>SIAGITEPTILQYFATLNAGEFAATAALFAVDGVMYPPFESGIVGPDAIAAYLQQEAQGIKAEPQQ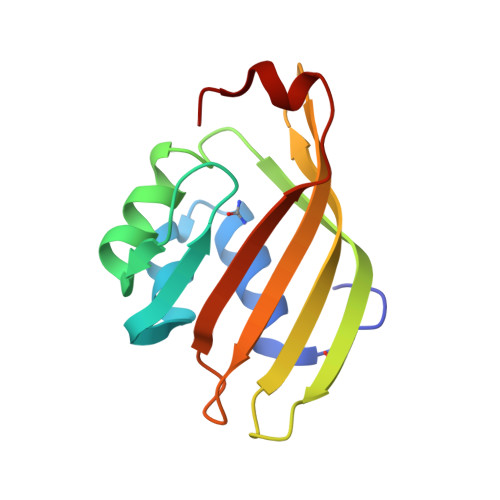GLAETSEDGHTQVQVSGKAQTSWCGVNVLWLFTLNQEKQIIHTQIKLLASPQELLALR[2x]> MGNTSIQTQSYRAVDKDAGQSRSYIIPFALLCSLFFLWAVANNLNDILLPQFQQAFTLTNFQAGLIQSAFYFGYFIIPIPAGILMKKLSYKAGIITGLFLYALGAALFWPAAEIMNYTLFLVGLFIIAAGLGCLETAANPFVTVLGPESSGHFRLNLAQTFASF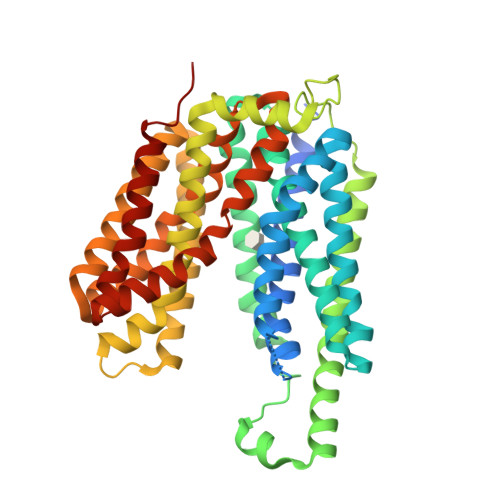GAIIAVVFGQSLILSNVPHQSQDVLDKMSPEQLSAYKHSLVLSVQTPYMIIVAIVLLVALLIMLTKFPALQSDNHSDAKQGSFSASLSRLARIRHWRWAVLAQFCYVGAQTACWSYLIRYAVEEIPGMTAGFAANYLTGTMVCFFIGRFTGTWLISRFAPHKVLAAYALIAMALCLISAFAGGHVGLIALTLCSAFMSIQYPTIFSLGIKNLGQDTKYGSSFIVMTIIGGGIVTPVMGFVSDAAGNIPTAELIPALCFAVIFIFARFRSQTATN>GPCSNHADSLNNLANIKREQGYIEEATRLYLKALEVFPDFAAAHSNLASVLQQQGKLKEALMHYKEAIRIQPTFADAYSNMGNTLKELQDVSGALQCYTRAIQINPAFADAHSNLASIHKDSGNIPEAIQSYRTALKLKPDFPDAYCNLAHCLQIVCDWTDYDIRMKKLVSIVTEQLEKNRLPSVHPHHSMLYPLTHDCRKAIAARHANLCLEKVHVLHKKPYNFLKKLPTKGRLRIGYLSSDFGNHPTSHLMQSVPGLHDRSKVEIFCYALSPDDGTTFRHKISRESENFVDLSQIPCNGKAADKIFNDGIHILVNMNGYTKGARNEIFALRPAPIQVMWLGYPGTSGASFMDYIITDSVTSPLELAYQYSEKLSYMPHTYFIGDHKQMFPHLKERIIVCDKQQSSVVDNVTVINATDLSPLVENTDVKEIKEVVNAQKPVEITHKVAELPNTTQIVSMIATGQVQTSLNGVVVQNGLATTQTNNKAATGEEVPQNIVITTRRQYMLPDDAVVYCNFNQLYMIDPQTLESWVEILKNVPKSVLWLLRFPAVGEQNIKKTVSDFGISPDRVIFSNVAAKEEHVRRGQLADICLDTPLCNGHTTSMDVLWTGTPVVTLPGETLASRVAASQLATLGCPELIARTREEYQN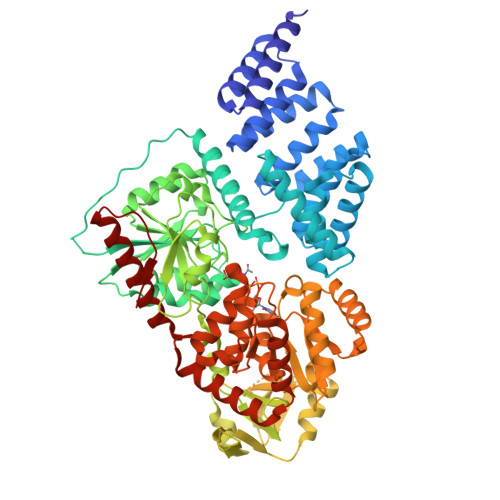IAIRLGTKKEYLKALRAKVWKARVESPLFDCSQYAKGLEKLFLRMWEKYENGELPDHISAV[3x]> AFVVTDNCIKCKYTDCVEVCPVDCFYEGPNFLVIHPDECIDDALCEPECPAQAIFSEDE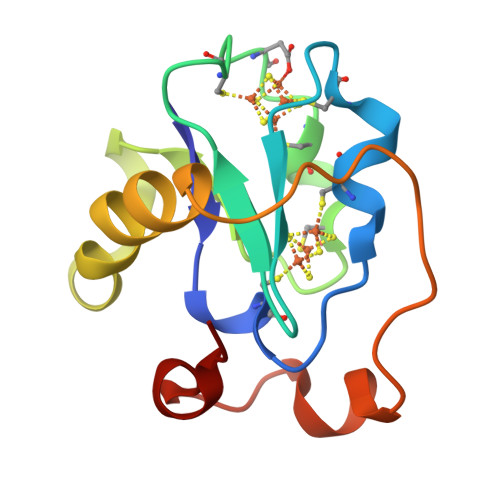VPEDMQEFIQLNAELAEVWPNITEKKDPLPDAEDWDGVKGKLQHLER> HKCDITLQEIIKDLNSLTEQKTLCTELTVTDIFAASKNTTEKETFCRAATVLRQFYSHHEKDTRCLGATAQQFHRHKQLIRDLKRLDRNLWGLAGLNSCPVKEANQSTLENFLE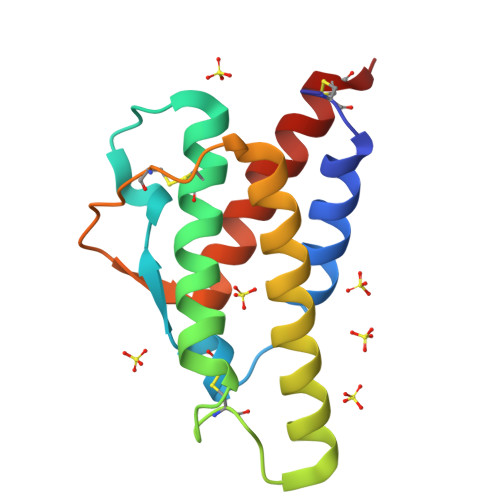RLKTIMREKYSKCSS>STQTAEDKEEPLHSIISSTESVQGSTSKHEFQAETKKLLDIVARSLYSEKEVFIRELISNASDALEKLRHKLVSDGQALPEMEIHLQTNAEKGTITIQDTGIGMTQEELVSNLGTIARSGSKAFLDALQNQAEASSKIIGQFGVGFYSAFMVADRVEVYSRSAAPGSLGYQWLSDGSGVFEIAEASGVRTGTKIIIHLKSDCKEFSSEARVRDVVTKYSNFVSFPLYLNGRRMNTLQAIWMMDPKDVREWQHEEFYRYVAQAHDKPRYTLHYKTDAPLNIRSIFYVPDMKPSMFDVSRELGSSVALYSRKVLIQTKATDILPKWLRFIRGVVDSEDIPLNLSRELL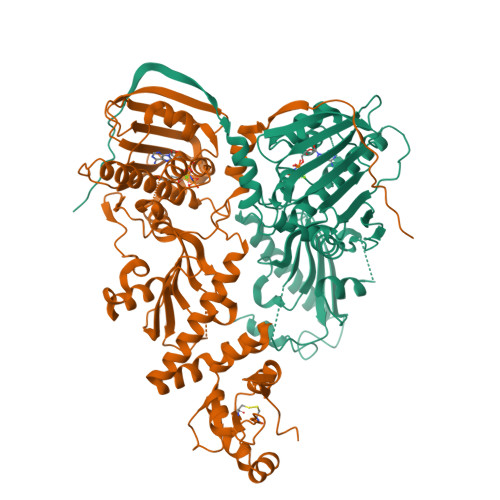QESALIRKLRDVLQQRLIKFFIDQSKKDAEKYAKFFEDYGLFMREGIVTATEQEVKEDIAKLLRYESSALPSGQLTSLSEYASRMRAGTRNIYYLCAPNRHLAEHSPYYEAMKKKDTEVLFCFEQFDELTLLHLREFDKKKLISVETDIVVDHYKE[4x]>[2x]MMNWEHLLSLKRQGDTAKRLRIEQDDTRLGFEVDYDRIIFSAPFRSLQDKTQVIPLSKTDFVHTRLTHSLEVSVVGRSLGRMVGKKLLEKYPHLEQV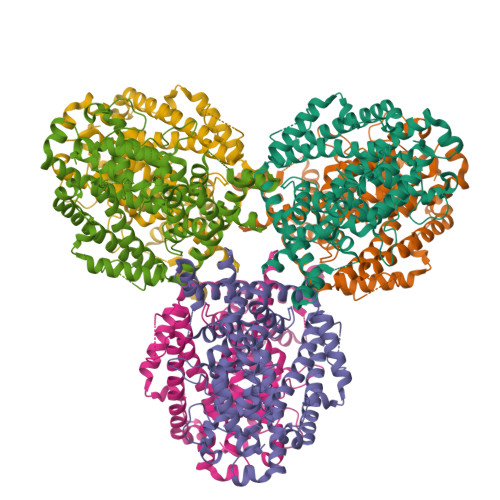YGYKFNDFGAIVAAAALAHDIGNPPFGHSGEKAIGEFFKNGYGKRYKDSLTAKEYQDLIKFEGNANGFKVLSQSKPGAQGGLRLSYATLGAFMKYPKESLPHKPSDHIADKKYGFFQSERALFEDVAQELGLLKRSTTDDVSWSRHPLAYLVEAADDICYTIIDFEDGINLGLIPEEYALEYMVKLVGQTIDRNKYNALQETSDRVSYLRALAIGTLINESVDTFMKYEEEILAGTFDQSLIDKSNYQAQITDIINLSIERIYNSREVIEKEIAGYEILSTLLEARCRALDNNDTHYNQLIQQLLAPNDHSEKSLYENLIQICAEVSTMTDGKALRNYKKIKGLDVK> HQAEVQIARKLQCIADQF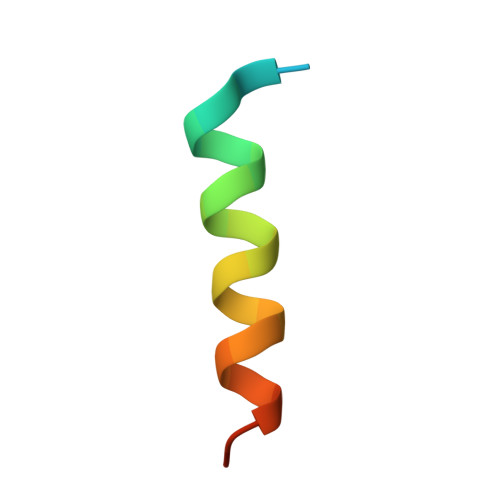HRLHVQQ> SNAMNRIDKTLEKLKANRKKMLSPYITAGDPYPELTVSLMHQLVKSGADVLELGIPFSDPMAEGPVIQRAMERALAHSIHCDDVLNMVRQFRKTDTETPVILMGYLNPIEQYGYDLFAQQAVEAGADGTILVDLP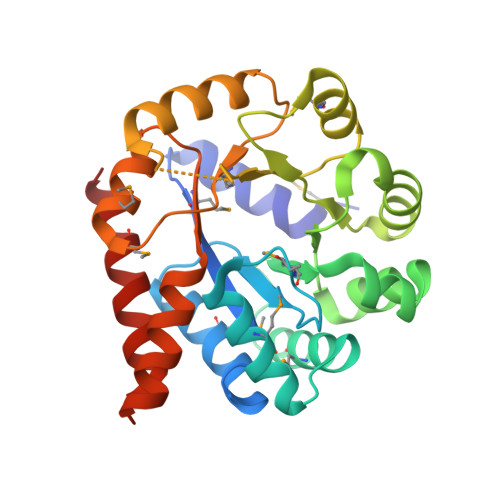PEEADGVSRVWQKHGLYSIYLCSPTTSAERMNFINQHANGYLYYVSLKGVTGSDALKLPELKAQYLQRKAQSKLPLMVGFGIKTPEMAAQVAEFADGVIVGAALINEIIEAYEAKKDPLQASGALLSSMRQAIDNIGSMV>[2x]SNAMKPKLILMSHGRMAEETLASTQMIVGELADAAIVSMTAEDGLSGTQAKLAAILKEAGNVPTLVLADLKGGTPCNVAMMAMGTY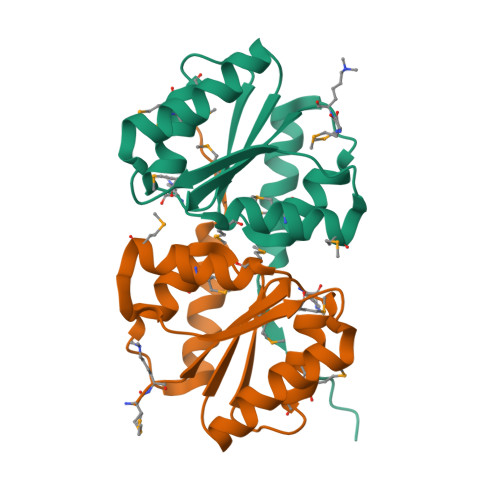PQLRVVAGLNLAMAIEAAVSPVENVDELAAYLTQIGQSAVTTIDLPELTDEEEFEE> QYTFIQKRTHLFACGIKRKSIKWICRENSEKITVCVPDRKIQLCIANFLNSRLETMEKFKEIFLISVNTEAKLLYNKNEGKDPSIFCNELRNSFSDFRNSFIGDDMDFGGNTDRVKGYINKKFSDYYKEKNVEKLNNIKKEWWEKNKANLWNHMIVNHKGNIAKECAIIPAEEPQINLWIKEWNENFLMEKKRLFLNIKDKCVENKKYEACFGGCRLPCSSYTSFMKKSKTQMEVLTNLYKKKNSGVDKNNFLNDLFKKNNKNDLDDFFKNEKEYDDLCDCRYTATIIKSFLNGPAKNDVDIASQINVNDLRGFGCNYKSNNEKSWNCAGTFTNKFPGTCEPPRRQTLCLGRTYLLHRGHEEDYKEHLLGASIYEAQLLKYKYKEKDENALCSIIQNSYADLADIIKGSDIIKDYYGKKMEENLNKVNKDKKRNEESLKIFREKWWDENKENVWKVMSAVLKNKETCKDYDKFQKI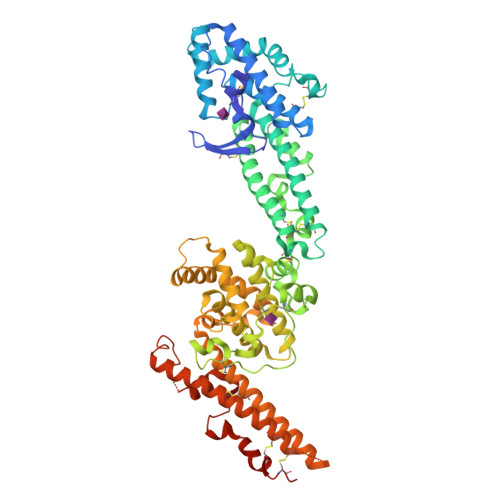PQFLRWFKEWGDDFCEKRKEKIYSFESFKVECKKKDCDENTCKNKCSEYKKWIDLKKSEYEKQVDKYTKDKNKKMYDNIDEVKNKEANVYLKEKSKECKDVNFDDKIFNEAPNEYEDMCKKCDEIKYLNEIKYPKTKHD> ETPPRFTRTPVDQTGVSGGVASFICQATGDPRPKIVWNKKGKKVSNQRFEVIEFDDGSGSVLRIQPLRTPRDEAIYECVASNNVGEISVSTRLTVLREDQIPRGFPTIDMGPQLKVVERTRTATMLCAASGNPDPEITWFKDFLPVDTSNNNGRIKQLRSESIGGTPIRGALQIEQSEESDQGKYECVATNSAGTRYSAPANLYVRELREVRRVPPRFSIPPTNHEIMPGGSVNITCVAVGSPMPYVKWMLGAEDLTPEDDMPIGRNVLELNDVRQSANYTCVAMSTLGVIEAIAQIT;> SADGCTDWSIDIKKYQVLVGEPVRIKCALFYGYIRTNYSLAQSAGLSLMWYKSSGPGDFEEPIAFDGSRMSKEEDSIWFRPTLLQDSGLYACVIRNSTYCMKVSISLTVGENDTGLCYNSKMKYFEKAELSKSKEISCRDIEDFLLPTREPEILWYKECRTKTWRPSIVFKRDTLLIREVREDDIGNYTCELKYGGFVVRRTTELTVTAPLTDKPPKLLYPMESKLTIQETQLGDSANLTCRAFFGYSGDVSPLIYWMKGEKFIEDLDENRVWESDIRILKEHLGEQEVSISLIVDSVEEGDLGNYSCYVENGNGRRHASVLL

The leukocyte common antigen-related receptor protein tyrosine phosphatases (LAR-RPTPs), including LAR, PTPσ and PTPδ in vertebrates, and dLAR in Drosophila, have recently emerged as a major family of synaptic adhesion molecules. Presynaptic LAR-RPTPs induce synaptic differentiation by binding several postsynaptic partners, including members of the Slit- and Trk-like family of proteins (Slitrks), interleukin-1 receptor accessory protein (IL-1RAcP), IL-1 receptor accessory protein-like 1 (IL1RAPL1), neurotrophin receptor tyrosine kinase C (TrkC), netrin-G ligand-3 (NGL-3), synaptic adhesion-like molecule 3 (SALM3) and synaptic adhesion-like molecule 5 (SALM5; Woo et al., 2009; Mah et al., 2010; Takahashi et al., 2011; Yoshida et al., 2011, 2012; Yim et al., 2013; Choi et al., 2016). LAR-RPTPs contain multiple splice sites—designated mini-exons A-D (MeA-D), that produce diverse LAR-RPTP variants with and without short peptide inserts. Recent progress in the structural characterization of trans-synaptic adhesion complexes, including LAR-RPTPs bound to Slitrks, TrkC, IL1RAPL1 or IL-1RAcP, have revealed the interaction interface of these complexes as well as the significant role of splice inserts, particularly that of MeA and MeB, in their selective binding.

Here, we determined the crystal structure of the human LAR-RPTP (PTPδ)/IL1RAPL1 complex and identified the lateral molecular interactions between neighboring LAR-RPTP (PTPδ)/IL1RAPL1 complexes in the crystal-packing lattices. Notably, these interactions were found to be essential for the formation of higher-order trans-synaptic adhesion complex assemblies (PTPδ/IL1RAPL1 complexes) and for IL1RAPL1-mediated presynaptic differentiation. Likewise, the binding of LAR-RPTPs to other postsynaptic adhesion molecules—Slitrk3 and IL-1RAcP (but not TrkC)—induces the formation of higher-order trans-synaptic adhesion complex assemblies. We also provide compelling evidence that HSPG, but not CSPG, inhibits the interactions of LAR-RPTPs with their postsynaptic ligands (Slitrk1, IL1RAPL1 and IL-1RAcP) and that HSPGs can even disrupt pre-established LAR-RPTP-mediated trans-synaptic adhesion complexes. Our results suggest that the competitive advantage of HSPGs over postsynaptic adhesion partners for LAR-RPTP binding can modulate LAR-RPTP-mediated synaptogenesis.D-MYO-INOSITOL-2,4,5-TRIPHOSPHATE | C6 H15 O15 P3 | 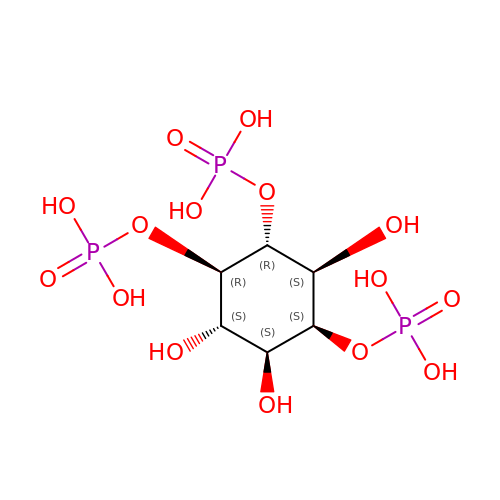MMWCIQZXVOZEGG-LKPKBOIGSA-N> AMRQCAIYGKGGIGKSTTTQNLVAALAEMGKKVMIVGCDPKADSTRLILHSKAQNTIMEMAAEAGTVEDLELEDVLKAGYGGVKCVESGGPEPGVGCAGRGVITAINFLEEEGAYEDDLDFVFYDVLGDVVCGGFAMPIRENKAQEIYIVCSGEMMAMYAANNISKGIVKYANSGSVRLGGLICNSRNTDREDELIIALANKLGTQMIHFVPRDNVVQRAEIRRMTVIEYDPKAKQADEYRALARKVVD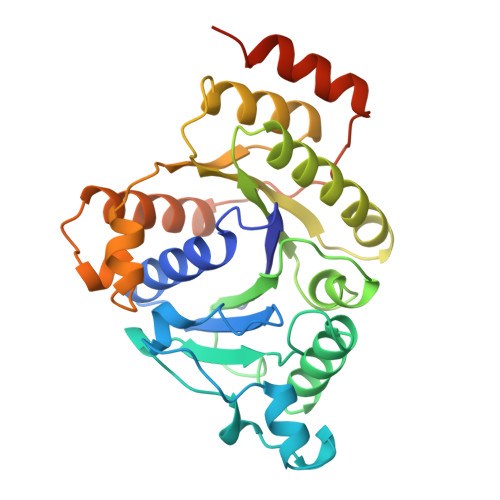NKLLVIPNPITMDELEELLMEFGIMEVEDESIVGKTAEEV8-n-octylamino-adenosine 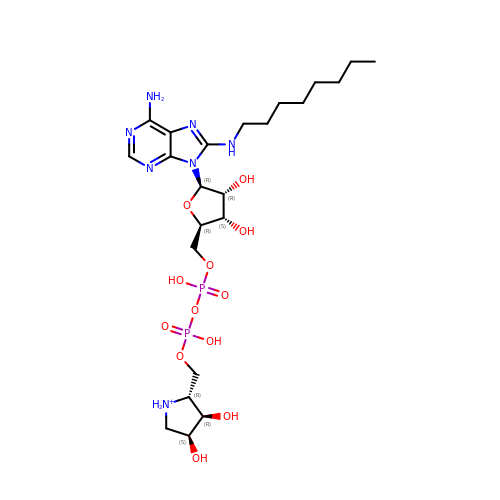diphosphate hydroxypyrrolidinediol | C23 H42 N7 O12 P2 | HQJQCBXMIIQUTE-WBZRXDBSSA-O propyl 2-(acetylamino)-4-O-{3-O-[(1-benzyl-1H-1,2,3-triazol-4-yl)methyl]-beta-D-galactopyranosyl}-2-deoxy-beta-D-glucopyranoside 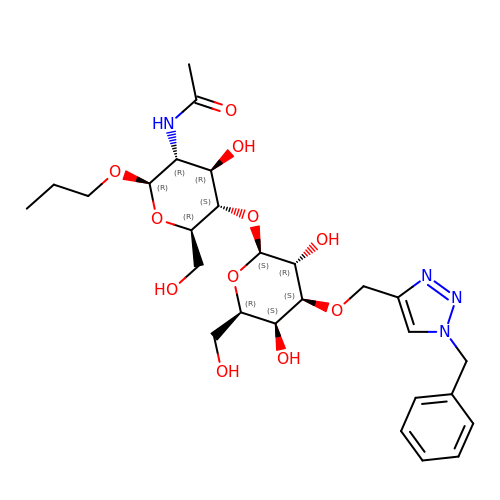| C27 H40 N4 O11 | GGSLGSZWTJXVOE-UNBRQLBDSA-N>[2x]MASQGPGEVVLLDFAAAGGELGWLTHPYGKGWDLMQNIMNDMPIYMYS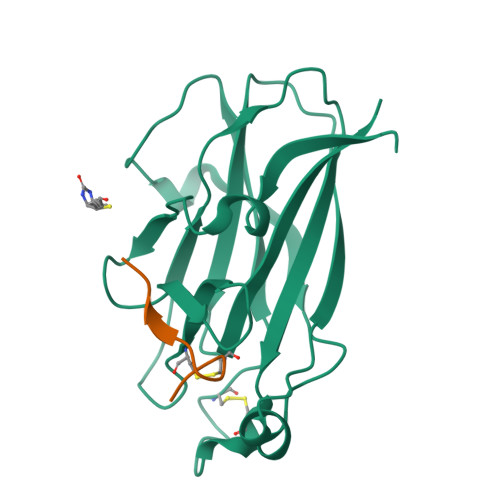VCNVMSGDQDNWLRTNWVYRGEAERIFIELKFTVRDCNSFPGGASSCKETFNLYYAESDLDYGTNFQKRLFTKIDTIAPDEITVSSDFEARHVKLNVEERSVGPLTRKGFYLAFQDIGACVALLSVRVYYKKAHHHHHH;>[2x]XWLAYPDSVPYSK>RLVQLSRHSIAFPSPEGALREPNGLLALGGDLSPARLLMAYQRGIFPWFSPGDPILWWSPDPRAVLWPESLHISRSMKRFHKRSPYRVTMNYAFGQVIEGCASDREEGTWITRGVVEAYHRLHELGHAHSIEVWREDELVGGMYGVAQGTLFC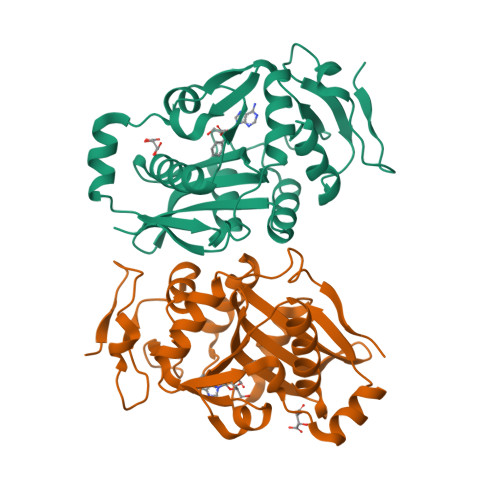GESMFSRMENASKTALLVFCEEFIGHGGKLIDCQVLNDHTASLGACEIPRRDYLNYLNQMRLGRLPNNFWVPRCLFSPQE[2x]>MRGSHHHHHHGSPSKVQELSVYEINELDRHSPKILKNAFSLMFGLGDLVPFTNKLYTGDLKKRVGITAGLCVVIEHVPEKKGERFEATYSFYFGDYGHLSVQGPYLTYEDSFLAITGGAGIFEGAYGQVKLQQLVYPTKLFYTFYLKGLANDLPLELTGTPVPPSKD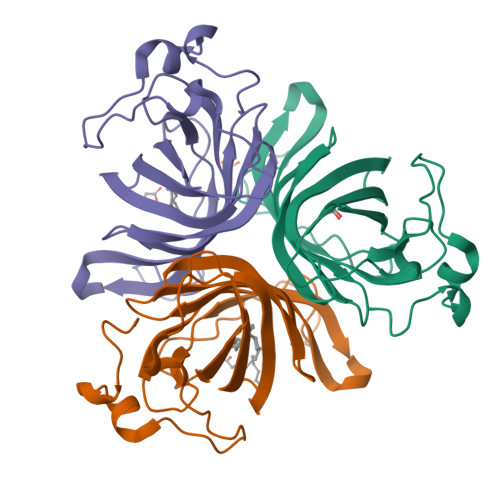IEPAPEAKALEPSGVISNYTN[3x]> MPEPTADAPTVPKARSCPFLPPDGIADIRAAAPVTRATFTSGHEAWLVTGYEEVRALLRDSSFSVQVPHALHTQDGVVTQKPGRGSLLWQDEPEHTSDRKLLAKEFTVRRMQALRPNIQRIVDEHLDAIEARGGPVDLVKTFANAVPS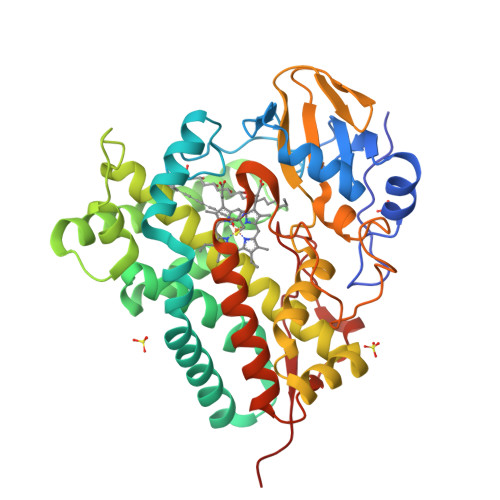MVISDLFGVPVERRAEFQDIAEAMMRVDQDAAATEAAGMRLGGLLYQLVQERRANPGDDLISALITTEDPDGVVDDMFLMNAAGTLLIAAHDTTACMIGLGTALLLDSPDQLALLREDPSLVGNAVEELLRYLTIGQFGGERVATRDVELGGVRIAKGEQVVAHVLAADFDPAFVEEPERFDITRRPAPHLAFGFGAHQCIGQQLARIELQIVFETLFRRLPGLRLAKPVEELRFRHDMVFYGVHELPVTWHHHH4-(2H-tetrazol-2-yl)-L-phenylalanine | C10 H11 N5 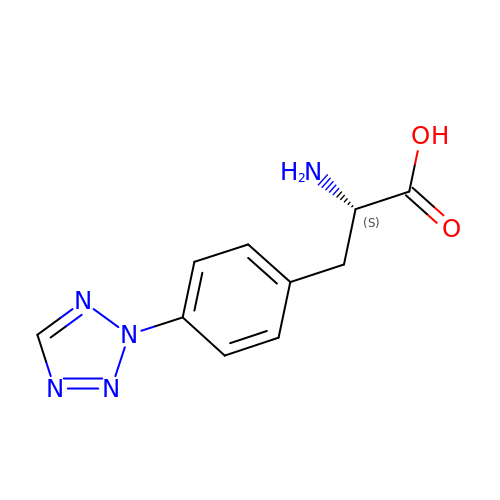O2 | KHTQUIIGXJUWFB-VIFPVBQESA-N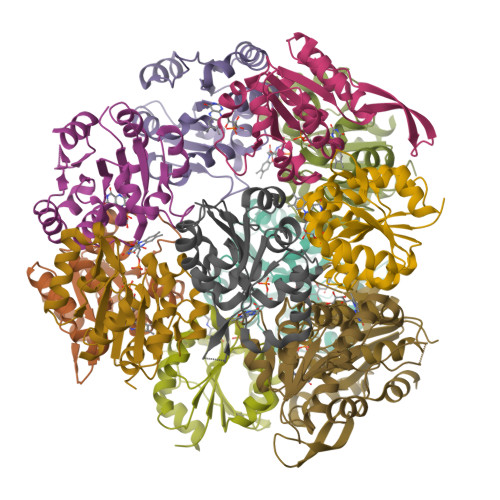>[12x]MYGKLLICATASINVININHYIVELKQHFDEVNILFSPSSKNFINTDVLKLFCDNLYDEIKDPLLNHINIVENHEYILVLPASANTINKIANGICDNLLTTVCLTGYQKLFIFPNMNIRMWGNPFLQKNIDLLKNNDVKVYSPDMNKSFEISSGRYKNNITMPNIENVLNFVLNNEKRPLD(2S)-2-{[4-(3-amino-4-methylphenyl)-6-methylpyrimidin-2-yl]oxy}-3-methoxy-3,3-diphenylpropanoic acid | C28 H27 N3 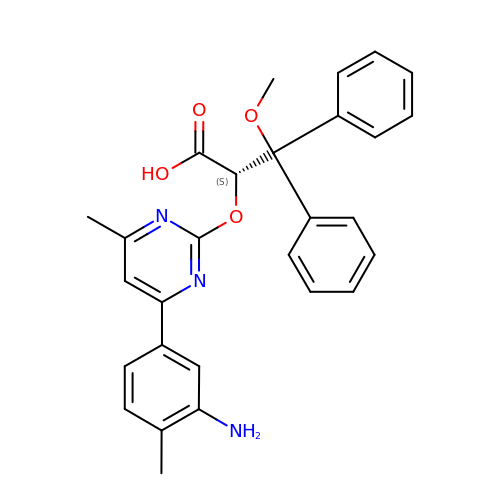O4 | GDPBXJYDHBGQBK-RUZDIDTESA-N4-bromo-N-(pyridin-2-ylmethyl)naphthalene-1-sulfonamide 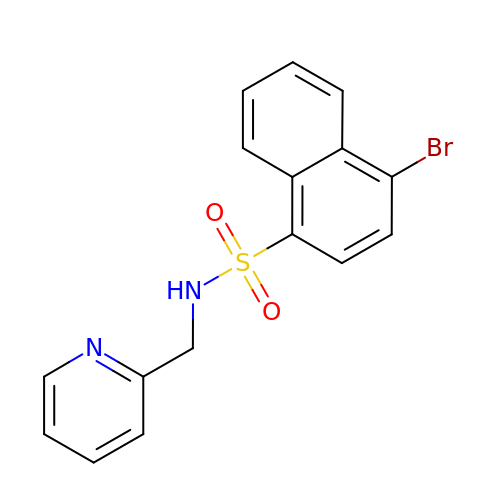| C16 H13 Br N2 O2 S | GJSDYQXOSHKOGX-UHFFFAOYSA-N(6R)-1-[4-[3-(dimethylamino)phenyl]-3,5-bis(fluoranyl)phenyl]-6-propan-2-yl-6,7-dihydro-5H-benzotriazol-4-one 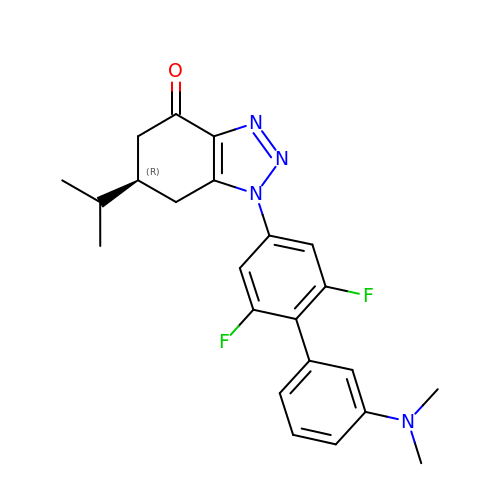| C23 H24 F2 N4 O | XGSICBDUCCZAFB-OAHLLOKOSA-N> GASGSGTGSGSMLYLIIYDVPATKAGNKRRTRLFDLLSGYGKWRQFSVFECF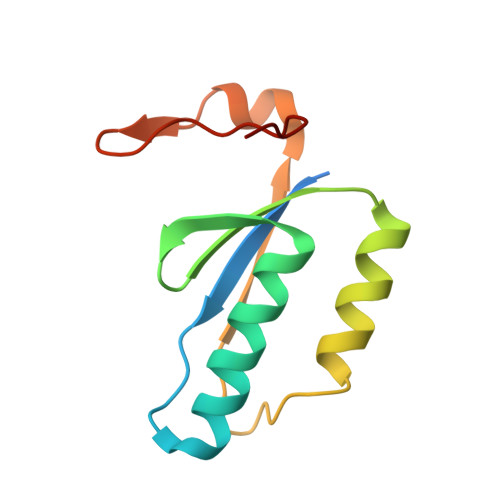LSVKQFAKLQTAMEKLIKLDEDAVCIYVLDENTVQRTITYGTPQPEKPGSIII(2~{S},3~{R})-2,6-bis(azanyl)-3-oxidanyl-hexanoic acid | C6 H14 N2 O3 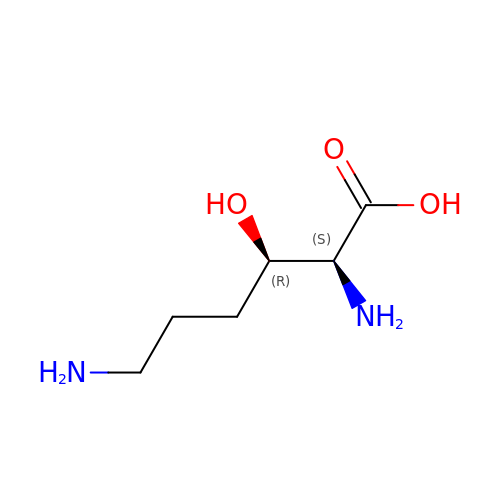| YSVMULOOWPBERR-UHNVWZDZSA-N> ATFLIWPIYPKIEANEKATAVWLQNTGKTDAMVQIRVFKWNQDGLKDNYSEQSEIIPSPPVAKIKAGEKHMLRLTKSVNLPDGKEQSYRLIVDELPIRLSDGNEQDASKVSFQMRYSIPLFAYGKGIGSGLTEESQKLNAKNALAKPVLQWSVRNNQQGQSELYLKNNGQKFARLSALKTSKTGNDISLGKAAFGYVLSNSTVKFAIDQSTAHELAKTSKIYGVDSSGIKQELIEITKMEDPS;> AVTHHHHHHSTGCTVGGSQTEGNMNKFGTLNFGKTSGTWNNVLTAEVASAATGGNISVTCDGTDPVDFTVAIDGGERTDRTLKNTASADVVAYNVYRDAAR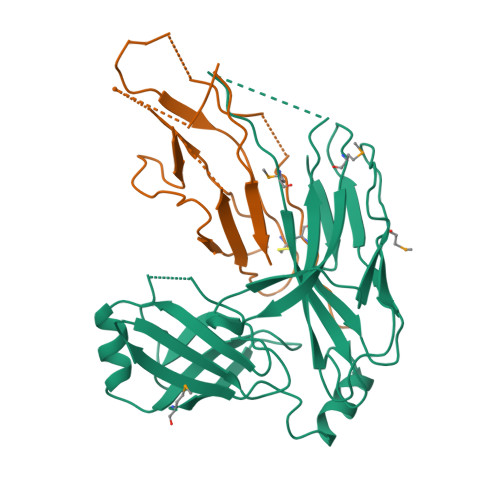TNLYVVNQPQQFTTVSGQATAVPIFGAIAPNTGTPKAQGDYKDTLLVTVNF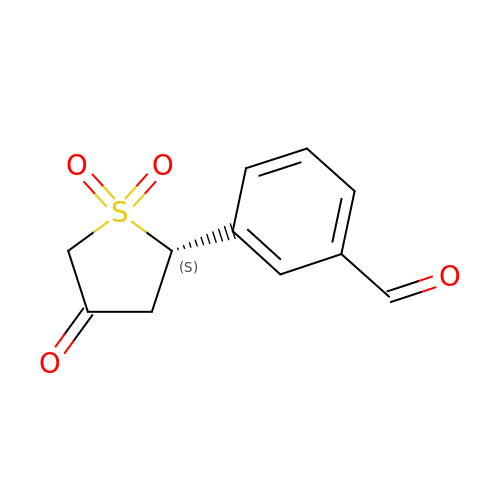3-[(2S)-1,1-DIOXIDO-4-OXOTETRAHYDROTHIOPHEN-2-YL]BENZALDEHYDE | C11 H10 O4 S | YIJQNPNARRVHGF-NSHDSACASA-N1-[4-[[(2~{S})-4-~{tert}-butylmorpholin-2-yl]methoxy]phenyl]-3-cyclohexyl-urea 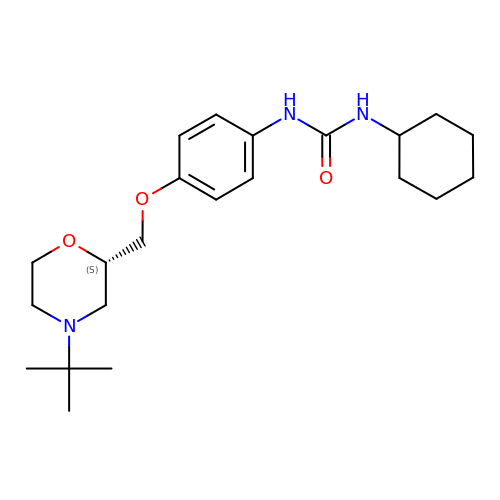| C22 H35 N3 O3 | PSVUAGRHPQWOOO-FQEVSTJZSA-N>[2x]GEGQDIWDMLDKGNPFQFYLTRVSGVKPKYNSGALHIKDILSPLFGTLVSSAQFNYCFDVDWLVKQYPPEFRKKPILLVHGDKREAKAHLHAQAKPYENISLCQAKLDIAFGTHHTKMMLLLYEEGLRVVIHTSNLIHA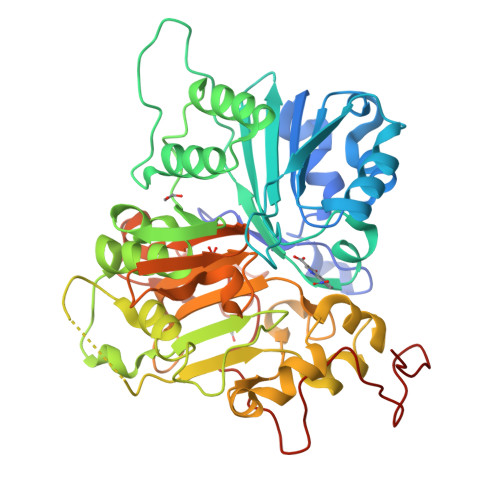DWHQKTQGIWLSPLYPRIADGTHKSGESPTHFKADLISYLMAYNAPSLKEWIDVIHKHDLSETNVYLIGSTPGRFQGSQKDNWGHFRLKKLLKDHASSMPNAESWPVVGQFSSVGSLGADESKWLCSEFKESMLTLGKESKTPGKSSVPLYLIYPSVENVRTSLEGYPAGGSLPYSIQTAEKQNWLHSYFHKWSAETSGRSNAMPHIKTYMRPSPDFSKIAWFLVTSANLSKAAWGALEKNGTQLMIRSYELGVLFLPSAFGLDSFKVKQKFFAGSQEPMATFPVPYDLPPELYGSKDRPWIWNIPYVKAPDTHGNMWVPS>DWAAVIPPINLPENSRGPFPQELV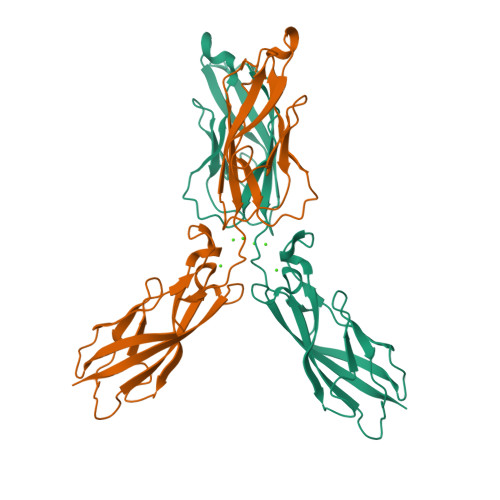RIRSDRDKNLSLRYSVTGPGADQPPTGIFIINPISGQLSVTKPLDRELIARFHLRAHAVDINGNQVENPIDIVINVIDMNDNRPEFLHQVWNGSVPEGSKPGTYVMTVTAIDADDPNALNGMLRYRILSQAPSTPSPNMFTINNETGDIITVAAGLDREKVQQYTLIIQATDMEGNPTYGLSNTATAVITVTD[3x]>SDSLSFSFINFDQDERNVIAQGDARISGNNILQLTRTDSDGTPVRSTVGRILYSAQVRLWEKSTNRVANFQSQFSFFLESPLSNPADGIAFFIAPPDTAIPSGSAGGLLGLFSPKTAQNESANQVLAVEFDTFYAQNSNTWDPNYPHIGIDVNSIKSAKTVRWERREGVTLNVLVTYNPSTKTLDVVATYPDGQRYQISVVVDVTTVL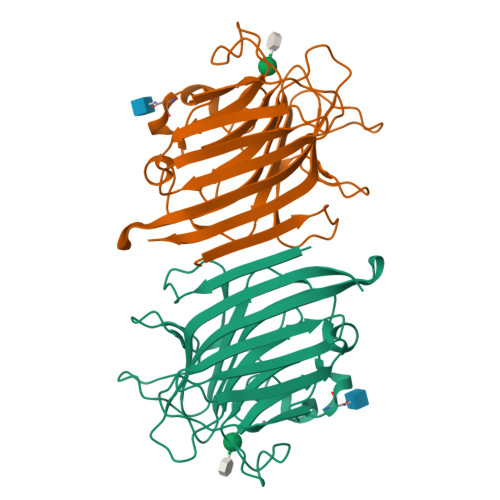PEWVRVGFSAASGEQFQTHNLESWSFTSTLLYTAQKE[2x]>MGSSHHHHHHSSGETVRFQGHMRNPAMYSEEARLKSFQNWPDYAHLTPRELASAGLYYTGIGDQVQCFACGGKLKNWEPGDRAWSEHR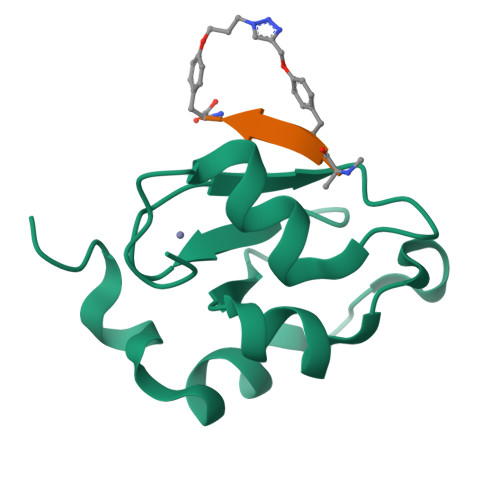RHFPNCFFVL[2x];>[2x]AFPFFX4-methyl-2-{[2-methyl-6-(methylsulfonyl)phenyl]amino}benzoic acid | C16 H17 N O4 S | 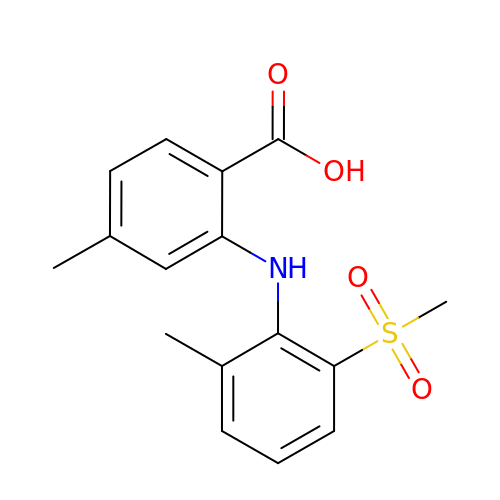ATXRRHMCJFBFND-UHFFFAOYSA-N>[2x]KPKLHYFNARGRMESTRWLLAAAGVEFEEKFIKSAEDLDKLRNDGYLMFQQVPMVEIDGMKLVQTRAILNYIASKYNLYGKDIKERALIDMYIEGIADLGEMILLLPVCPPEEKDAKLALIKEKIKNRYFPAFEKVLKSHGQDYLVGNKLSRADIHLVELLYYVEELDSSLISSFPLLKALKTRISNLPTVKKFLQPGSPRKPPMDEKSLEEARKIF

Glutathione transferases (GSTs) are a family of Phase II detoxification enzymes that catalyse the conjugation of the tripeptide glutathione (γ-Glu-Cys-Gly, GSH) to a wide variety of electrophilic compounds. Structural studies have shown that GSTs are dimeric enzymes with each subunit containing a GSH-binding site (G-site) and a second adjacent hydrophobic binding site for the electrophilic substrate (H-site). Human GSTA1-1 (hGSTA1-1) is an effective catalyst for chlorambucil conjugation with GSH. The active hGSTA1-1 enzyme is a homodimer.

The hGSTA1-1 enzyme was crystallized in the presence of CBL and the X-ray crystal structure was determined by molecular replacement at 2.1 Å resolution. Difference Fourier electron density maps indicate the presence of a GSH moiety in the G-site of the enzyme. Specifically it forms a salt bridge with Arg131 and hydrogen bonds with the side chains of Thr68 and Asp101 and the main chain carbonyl of Val55. Electron density is observed indicating the presence of a chemical moiety in the H-site that is attached to the thiol group of GSH that is bound to both monomers. The electron density feature is more prominent for the binding site of monomer A and has a shape consistent with a portion of the CBL moiety, conjugated with bound GSH. For both monomers, there is no electron density for the carboxylate moiety of CBL and for monomer B, the remaining CBL density becomes progressively poorer going from the thiol group to the aromatic ring of CBL. These may be consequences of the high mobility of the CBL moiety due to its extensive exposure to the solvent and lack of specific interactions. Comparison of the structure with those of previously reported hGSTA1-1/GSH complexes shows very few differences in the position of the GSH atoms with the exception of the thiol group of GSH which rotates in order to accommodate the bond with the CBL moiety. Several van der Waals and hydrophobic contacts exist between the CBL moiety and several residues including Gly14, Leu107, Leu108, Val111, Met208 and Phe220. Comparison of the two structures shows few differences in the position of the protein side chains, with the exception of Phe10 side chain which rotates in order to form van der Waals contacts with the aromatic ring of CBL and significant differences in the positions of C-helix residues, in particular that of Met208.> MIPAALPHPTMKRQGDRDIVVTGVRNQFATDLEPGGSVSCMRSSLSFLSLLFDVGPRDVLSAEAIEGCLVEGGEWTRAAAGSGPPRMCSIIELPNFLEYPAARGGLRCVFSRVYGEVGFFGEPTAGLLETQCPAHTFFAGPWAMRPLSYTLLTIGPLGMGLYRDGDTAYLFDPHGLPAGTPAFIAKVRAGDVYPYLTYYAHDRPKVRWAGAMVFFVPSGPGAVAPADLTAAALHLYGASETYLQDEPFVERRVAITHPLRGEIGGLGALFVGVVPRGDGEGSGPVVPALPAPTHVQTPGADRPPEAPRGASGPPDTPQAGHPNRPPDDVWAAALEGTPPAKPSAPDAAASGPPHAAPPPQTPAGDAAEEAEDLRVLEVGAVPVGRHRARYSTGLPKRRRPTWTPPSSVEDLTSGERPAPKAPPAKAKKKSAPKKKAPVAAEVPASSPTPIAATVPPAPDTPPQSGQGGGDDGPASPSSPSVLETLGARRPPEPPGADLAQLFEVHPNVAATAVRLAARDAALAREVAACSQLTINALRSPYPAHPGLLELCVIFFFERVLAFLIENGARTHTQAGVAGPAAALLDFTLRMLPRKTAVGDFLASTRMSLADVAAHRPLIQHVLDENSQIGRLALAKLVLVARDVIRETDAFYGDLADLDLQLRAAPPANLYARLGEWLLERSRAHPNTLFAPATPTHPEPLLHRIQALAQFARGEEMRVEAEAREMREALDALARGVDSVSQRAGPLTVMPVPAAPGAGGRAPCPPALGPEAIQARLEDVRIQARRAIESAVKEYFHRGAVYSAKALQASDSHDCRFHVASAAVVPMVQLLESLPAFDQHTRDVAQRAALPPPPPLATSPQAILLRDLLQRGQPLDAPEDLAAWLSVLTDAATQGLIERKPLEELARSIHGINDQQARRSSGLAELQRFDALDAALAQQLDSDAAFVPATGPAPYVDGGGLSPEATRMAEDALRQARAMEAAKMTAELAPEARSRLRERAHALEAMLNDARERAKVAHDAREKFLHKLQGVLRPLPDFVGLKACPAVLATLRASLPAGWTDLADAVRGPPPEVTAALRADLWGLLGQYREALEHPTPDTATALAGLHPAFVVVLKTLFADAPETPVLVQFFSDHAPTIAKAVSNAINAGSAAVATASPAATVDAAVRAHGALADAVSALGAAARDPASPLSFLAVLADSAAGYVKATRLALEARGAIDELTTLGSAAADLVVQARRACAQPEGDHAALIDAAARATTAARESLAGHEAGFGGLLHAEGTAGDHSPSGRALQELGKVIGATRRRADELEAAVADLTAKMAAQRARGSSERWAAGVEAALDRVENR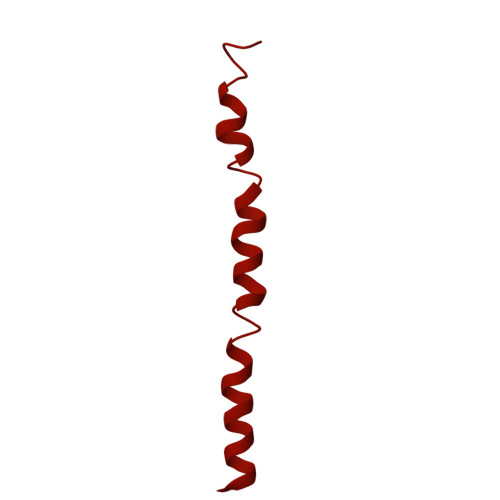AEFDVVELRRLQALAGTHGYNPRDFRKRAEQALAANAEAVTLALDTAFAFNPYTPENQRHPMLPPLAAIHRLGWSAAFHAAAETYADMFRVDAEPLARLLRIAEGLLEMAQAGDGFIDYHEAVGRLADDMTSVPGLRRYVPFFQHGYADYVELRDRLDAIRADVHRALGGVPLDLAAAAEQISAARNDPEATAELVRTGVTLPCPSEDALVACAAALERVDQSPVKNTAYAEYVAFVTRQDTAETKDAVVRAKQQRAEATERVMAGLREALAARERRAQIEAEGLANLKTMLKVVAVPATVAKTLDQARSVAEIADQVEVLLDQTEKTRELDVPAVIWLEHAQRTFETHPLSAARGDGPGPLARHAGRLGALFDTRRRVDALRRSLEEAEAEWDEVWGRFGRVRGGAWKSPEGFRAMHEQLRALQDTTNTVSGLRAQPAYERLSARYQGVLGAKGAERAEAVEELGARVTKHTALCARLRDEVVRRVPWEMNFDALGGLLAEFDAAAADLAPWAVEEFRGARELIQYRMGLYSAYARAGGQTGAGAESAPAPLLVDLRALDARARASSSPEGHEVDPQLLRRRGEAYLRAGGDPGPLVLREAVSALDLPFATSFLAPDGTPLQYALCFPAVTDKLGALLMRPEAACVRPPLPTDVLESAPTVTAMYVLTVVNRLQLALSDAQAANFQLFGRFVRHRQATWGASMDAAAELYVALVATTLTREFGCRWAQLGWASGAAAPRPPPGPRGSQRHCVAFNENDVLVALVAGVPEHIYNFWRLDLVRQHEYMHLTLERAFEDAAESMLFVQRLTPHPDARIRVLPTFLDGGPPTRGLLFGTRLADWRRGKLSETDPLAPWRSALELGTQRRDVPALGKLSPAQALAAVSVLGRMCLPSAALAALWTCMFPDDYTEYDSFDALLAARLESGQTLGPAGGREASLPEAPHALYRPTGQHVAVLAAATHRTPAARVTAMDLVLAAVLLGAPVVVALRNTTAFSRESELELCLTLFDSRPGGPDAALRDVVSSDIETWAVGLLHTDLNPIENACLAAQLPRLSALIAERPLADGPPCLVLVDISMTPVAVLWEAPEPPGPPDVRFVGSEATEELPFVATAGDVLAASAADADPFFARAILGRPFDASLLTGELFPGHPVYQRPLADEAGPSAPTAARDPRDLAGGDGGSGPEDPAAPPARQADPGVLAPTLLTDATTGEPVPPRMWAWIHGLEELASDDAGGPTPNPAPALLPPPATDQSVPTSQYAPRPIGPAATARETRPSVPPQQNTGRVPVAPRDDPRPSPPTPSPPADAALPPPAFSGSAAAFSAAVPRVRRSRRTRAKSRAPRASAPPEGWRPPALPAPVAPVAASARPPDQPPTPESAPPAWVSALPLPPGPASARGAFPAPTLAPIPPPPAEGAVVPGGDRRRGRRQTTAGPSPTPPRGPAAGPPRRLTRPAVASLSASLNSLPSPRDPADHAAAVSAAAAAVPPSPGLAPPTSAVQTSPPPLAPGPVAPSEPLCGWVVPGGPVARRPPPQSPATKPAARTRIRARSVPQPPLPQPPLPQPPLPQPPLPQPPLPQPPLPQPPLPQPPLPQPPLPQPPLPQPPLPPVTRTLTPQSRDSVPTPESPTHTNTHLPVSAVTSWASSLALHVDSAPPPASLLQTLHISSDDEHSDADSLRFSDSDDTEALDPLPPEPHLPPADEPPGPLAADHLQSPHSQFGPLPVQANAVLSRRYVRRTGRSALAVLIRACRRIQQQLQRTRRALFQRSNAVLTSLHHVRMLLG> MEPHSLRYNLTVLSWDGSVQSGFL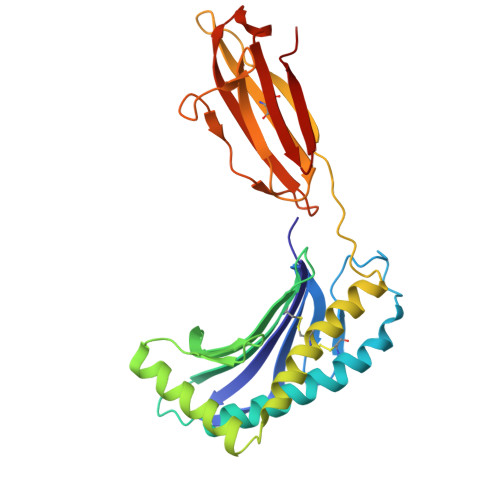TEVHLDGQPFLRCDRQKCRAKPQGQWAEDVLGNKTWDRETRDLTGNGKDLRMTLAHIKDQKEGLHSLQEIRVCEIHEDNSTRSSQHFYYDGELFLSQNLETKEWTMPQSSRAQTLAMNVRNFLKEDAMKTKTHYHAMHADCLQELRRYLKSGVVLRRTVPPMVNVTRSEASEGNITVTCRASGFYPWNITLSWRQDGVSLSHDTQQWGDVLPDGNGTYQTWVATRICQGEEQRFTCYMEHSGNHSTHPVPS> DRVYIHPFHLVIHNESTCEQLAKANAGKPKDPTFIPAPIQAKTSPVDEKALQDQLVLVAAKLDTEDKLRAAMVGMLANFLGFRIYGMHSELWGVVHGATVLSPTAVFGTLASLYLGALDHTADRLQAILGVPWKDKQCTSRLDAHKVLSALQAVQGLLVAQGRADSQAQLLLSTVVGVFTAPGLHLKQPFVQGLALYTPVVLPRSLDFTELDVAAEKIDRFMQAVTGWKTGSSLMGASVDSTLAFNTYVHFQGKMKGFSLLAEPQEFWVDQSTSVSVPMLSGMGTFQHWSDIQDQFSVTQVPFTESASLLLIQPHYASDLDKVEGLTFQQNSLNWMKKLSPRTIHLTMPQLVLQGSYDLQDLLAQAELPAILHTELNLQKLSNDRIRVGEVLNSIFFELEADEREPTESTQQLNKPEVLEVTLNRPFLFAVYDQSATALHFLGRVANPLSTAHHHHHH

Human blood pressure is mainly controlled by the renin–angiotensin system, which consists of several key components, including renin, angiotensinogen (AGT),3 angiotensin-converting enzyme (ACE), and angiotensin receptors. Renin is a highly specific aspartic protease that cleaves AGT between Leu10 and Val11 to release the N-terminal angiotensin I peptide. Cleavage of AGT by renin is the rate-limiting step of the renin–angiotensin system. To address these questions, here we have solved high-resolution crystal structures of human glycosylated AGT, its encounter complex with renin, AGT cleaved in the reactive center loop, and the spent AGT from which the N-terminal angiotensin peptide has been removed by renin.

Subsequently, we prepared spent AGT, where the N-terminal 10-residue angiotensin I peptide was removed from the AGT-N14 expression construct and loop-cleaved AGT, where AGT-N14 was cleaved between Gln412 and Leu413 by thermolysin treatment. To confirm conclusions from biochemical experiments that cleavage of the reactive center loop of AGT does not trigger the stressed-to-relaxed (S-to-R) transition characteristic of inhibitory serpins, we solved the structure of AGT cleaved by thermolysin treatment and compared it with that of intact AGT. Loop cleavage indeed induces no significant conformational changes, with an r.m.s. deviation of only 0.28 Å over 371 Cα atoms. The cleaved loop is disordered, but is not inserted into the central β-sheet A. In contrast, it has been shown that AGT has lost the ability to undergo this typical serpin S-to-R transition, confirmed here by our structure of loop-cleaved AGT, so it was very puzzling why the serpin framework was selected in the course of evolution as an angiotensin carrier.9-ethyl-8-ethynyl-purin-6-amine | C9 H9 N5 | 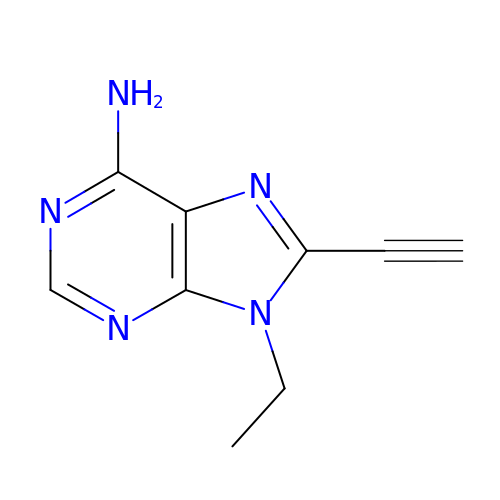AZRUGQVPCIZUAB-UHFFFAOYSA-N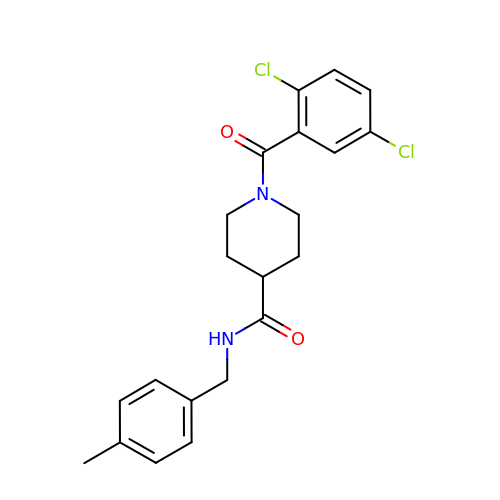1-[2,5-bis(chloranyl)phenyl]carbonyl-~{N}-[(4-methylphenyl)methyl]piperidine-4-carboxamide | C21 H22 Cl2 N2 O2 | HWTLZRSGBYUJIG-UHFFFAOYSA-N> MDPTISVSKGCFVYKNGATRAGKKAASKRKRPAAESSSLLGKEVVQQPFYEEYRKAWNQINDHIADLQHRSYARTLEQLVDFVVGQAERDTPDEVLPTAALLTGINQPDHLSQFTALTQRLHAQRAAMVCVLQSRDCATLKAAVETLVFGLVEDNAEVEQMEDEDEDEDGAERDRKRLRRSQCTMKQLKSWYTNNFDSEQKRRQLVVILPDFECFNASVLQDLILILSAHCGSLPFVLVLGVATAMTAVHGT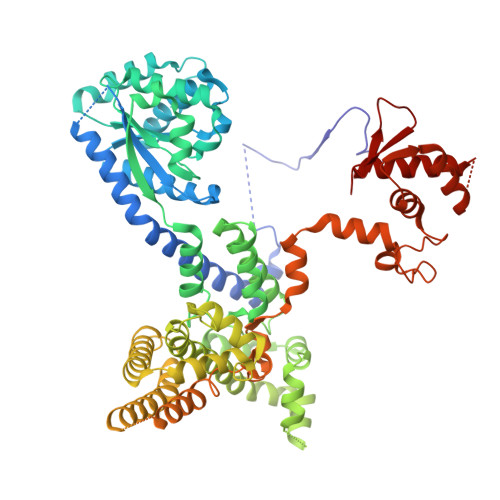LPYHVSSKIRLRVFQTQAAPTGLNEVLDKVLLSPKYAFHLSGKTFKFLTHIFLYYDFSIHGFIQGFKYCLMEHFFGGNAFALCTDYSKALGRIKQLTHEDMETIRRLPSFRPYVEQINDCKRIIAVLTDDDYLKKKLPQLLRDCLLHFLLFRCSLEFLTELVGDLPRCPLGKLRRELYVNCLNRAIISTPEYKECLQMLSFLSKDEFVAKVNRALERTEQFLVEEIAPLELGEACTAVLRPKLEAIRLAVDEVVKATMATITTTSPNETRQATDHLTPVASRQELKDQLLQRSKEDKMRHQLNTPTTQFGRALQKTLQLIETQIVQDHLRALQDAPPIHELFVFSDIATVRRNIIGAPRAALHTALNNPHFYMQCKCCELQDQSLLVGTLPDLSVVYKLHLECGRMINLFDWLQAFRSVVSDSDHEEVAQEQIDPQIQARFTRAVAELQFLGYIKMSKRKTDHATRLTW> MGSSHHHHHHLEVLFQGPHMSGVKVRREDAKKVLELL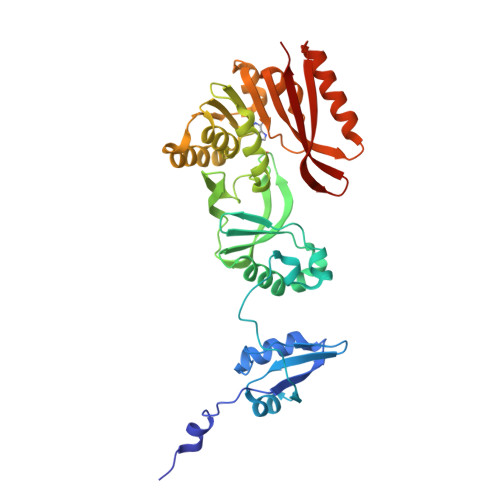KSVGILDGKRKAIRDEKYVIFPVTDTNIAKSLGLEVVDVELPMRPERQIYKNLEDLLPREIFKKLGRLDIVGDIAIVSIPDEILSEREVIVSAIRKLYPKVKVIARRGFHSGLYRIRELEVIWGENRLHTIHKENGVLIKVDLSKVFFNPRMKGERYRIAQLVNDGERILVPFAGVIPYPLVIARFKNVEVYAVEINEFAVKLAEENLELNRDRLKGKIKIIHGDVFEVLPNLPNFDRVVSPTPKGVDALSLTLSKAEKFLHYYDFVHESEIERFRERVLEECRRQGKECRVSVRKVSDYKPHVYKVCADVEILS> MAFELFTPLFNKIDQTTATYVTDISSRAIAAITPVVSVGLTLGFITYGWLIIRGAVEMPVAEFLNRCLRIGIIVSIALAGGLYQGEIANAITTVPDELASALLGNPTQGASAAALVDQSAQQGFDRASEAFEEAGFFSSDGLLYGLFGIIILLATGLLAAIGGAFLLLAKIALALLAGLGPLFILALIWQPTHRFFDQWAQQVLNYGLLIVLFAAVFGLLMQ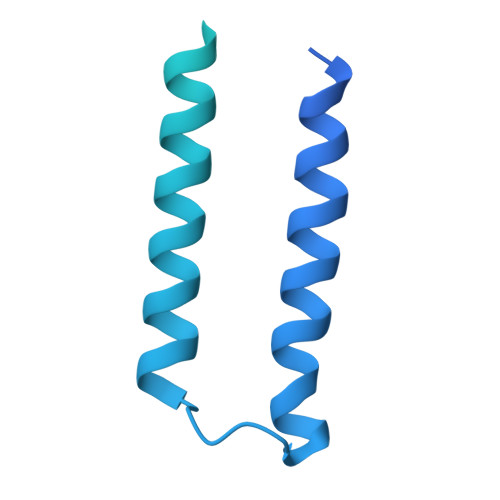IFGSYMADLRFDGAQNVAYAIGGSVILSIVSIVLLMQLPSIASGLAGGIGLGYMWELRSMRSGAGAAMRGGRAMARGARAAPGAARGAAVGAANMAKTVATGGAGVARAAAGYFRGRKAG> PFFVNRG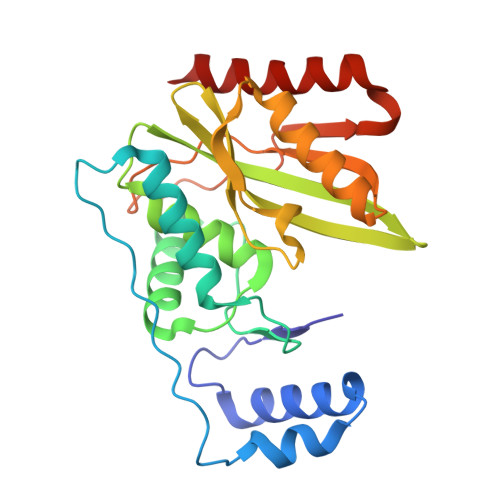GLPVDEATWERMWKHVAKIHPDGEKVAQRIRGATDLPKIPIPSVPTFQPSTPVPERLEAVQRYIRELQYNHTGTQFFEIKKSRPLTGLMDLAKEMTKEALPIKCLEAVILGIYLTNSMPTLERFPISFKTYFSGNYFRHIVLGVNFAGRYGALGMSRREDLMYKPPAFRTLSELVLDFEAAYGRCWHVLKKVKLGQSVSHDPHSVEQIEWKHSVLDVERLGRDDFRKELERHARDMRLKI(1R,2S)-2-(4-[cyclohexyl(2-methylpropyl)amino]-3-{[(4-methylphenyl)carbamoyl]amino}phenyl)cyclopropane-1-carboxylic acid | C28 H37 N3 O3 | 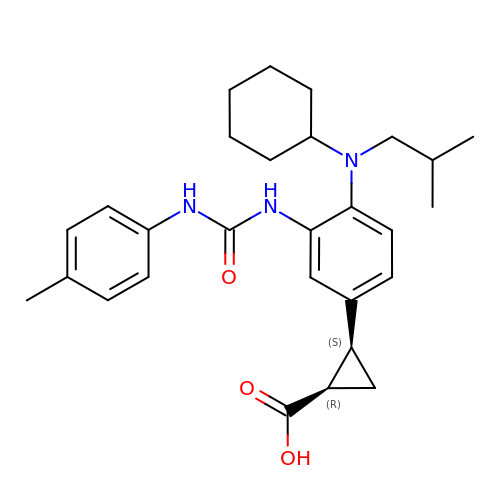AHNMZQOTEVUTJH-DNQXCXABSA-N>GAMWHTHSEREKRVSNAVE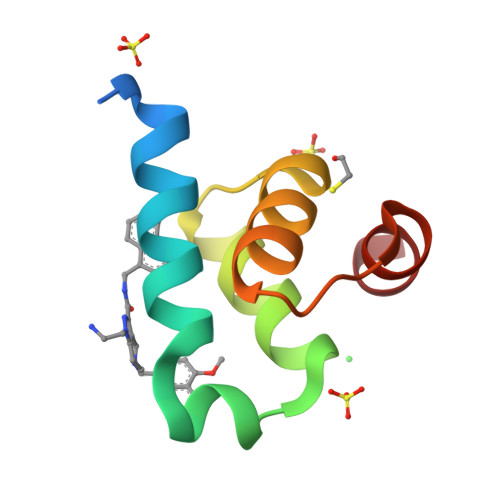FLLDSRVRRTPTSSKVHFLKSKGLSAEEICEAFTKVGQPKTLNEIKRILS[4x]> SVVTVRVQYLEDTDPFACANFPEPRRAPTCSLDGALPLG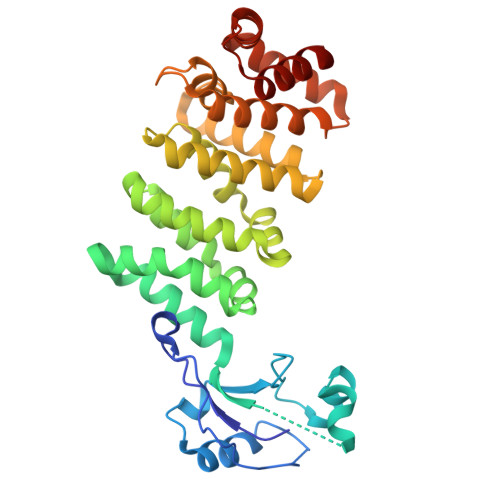AQIPAVHRLLGAPLKLEDCALQVSPSGYYLDTELSLEEQREMLEGFYEEISKGRKPTLILRTQLSVRVNAILEKLYSSSGPELRRSLFSLKQIFQEDKDLVPEFVHSEGLSCLIRVGAAADHNYQSYILRALGQLMLFVDGMLGVVAHSDTIQWLYTLCASLSRLVVKTALKLLLVFVEYSENNAPLFIRAVNSVASTTGAPPWANLVSILEEKNGADPELLVYTVTLINKTLAALPDQDSFYDVTDALEQQGMEALVQRHLGTAGTDVDLRTQLVLYENAL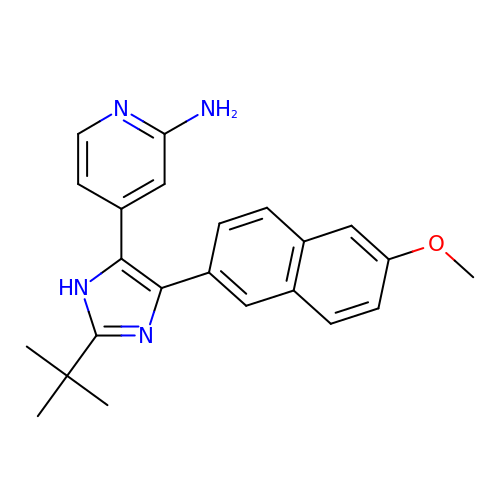4-(2-TERT-BUTYL-4-(6-METHOXYNAPHTHALEN-2-YL)-3H-IMIDAZOL-4-YL)PYRIDIN-2-AMINE | C23 H24 N4 O | KTHRIEHJGYTJED-UHFFFAOYSA-N>[6x]GSGSGSGMEKTQETVQRILLEPYKYLLQLPGKQVRTKLSQAFNHWLKVPEDKLQIIIEVTEMLHNASLLIDDIEDNSKLRRGFPVAHSIYGIPSVINSANYVYFLGLEKVLTLDHQDAVKLFTRQLLELHQGQGLDIYWRDNYTCPTEEEYKAMVLQKTGGLFGLAVGLMQLF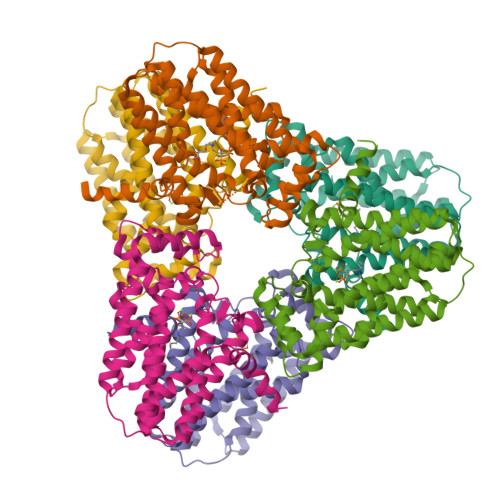SDYKEDLKPLLNTLGLFFQIRDDYANLHSKEYSENKSFCEDLTEGKFSFPTIHAIWSRPESTQVQNILRQRTENIDIKKYCVHYLEDVGSFEYTRNTLKELEAKAYKQIDARGGNPELVALVKHLSKMFKEENE(3R)-3-(cyclohexylcarbonylamino)-2-oxidanyl-3,4-dihydro-1,2-benzoxaborinine-8-carboxylic 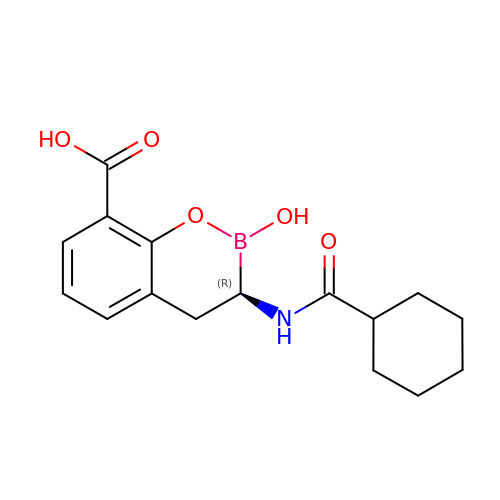acid | C16 H20 B N O5 | ZRHUJXRVIMMHFG-ZDUSSCGKSA-N> MEPTRIATNDRLSAAVCFDALVFLSGQVPGQAEDIHGQTREVLAKID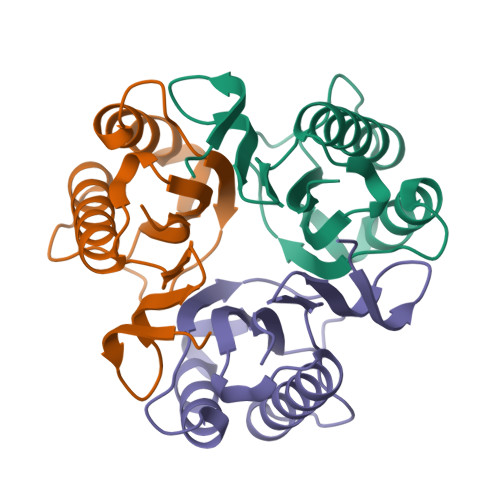ALLAEAGSRKERILSATIYLKDIARDFAALNEVWTQWLPTGQAPSRTTVQAELARPSVLVEITVVAARG> MKTPTIPTLLGPDGMTSLREYAGYHGGGSGFGGQLRSWNPPSESVDAALLPNFTRGNARADDLVRNNGYAANAIQLHQDHIVGSFFRLSHRPSWRYLGIGEEEARAFSREVEAAWKEFAEDDCCCIDVERKRTFTMMIREGVAMHAFNGELFVQATWDTSSSRLFRTQFRMVSPKRISNPNNTGDSRNCRAGVQINDSGAALGYYVSEDGYPGWMPQKWTWIPRELPGG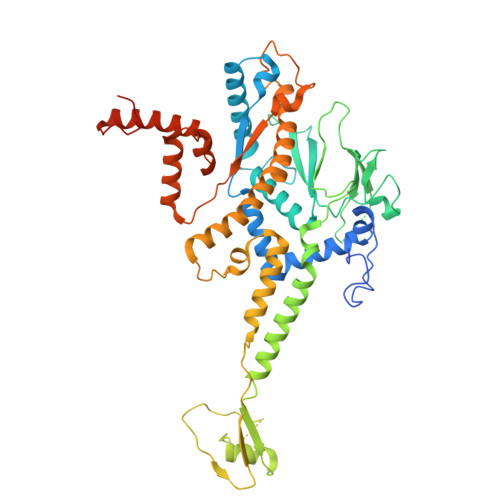RASFIHVFEPVEDGQTRGANVFYSVMEQMKMLDTLQNTQLQSAIVKAMYAATIESELDTQSAMDFILGANSQEQRERLTGWIGEIAAYYAAAPVRLGGAKVPHLMPGDSLNLQTAQDTDNGYSVFEQSLLRYIAAGLGVSYEQLSRNYAQMSYSTARASANESWAYFMGRRKFVASRQASQMFLCWLEEAIVRRVVTLPSKARFSFQEARSAWGNCDWIGSGRMAIDGLKEVQEAVMLIEAGLSTYEKECAKRGDDYQEIFAQQVRETMERRAAGLKPPAWAAAAFESGLRQSTEEEKSDSRAA>[2x]ADPEVRRCSEQRCPAPYEICPEDYLMSMVWKRTPAGDLAFNQCPLNATGTTSRRCSLSLHGVAFWEQPSFARCISNEYRHLQHSI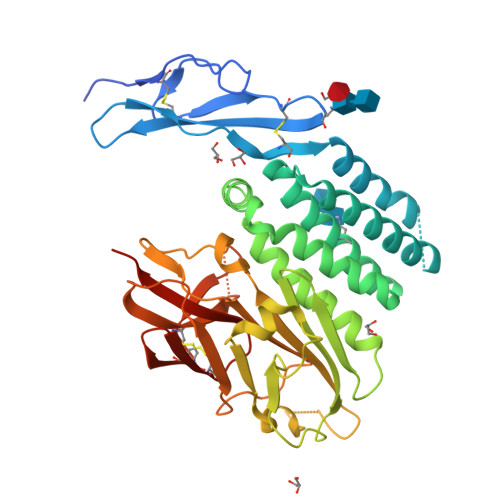KEHLAKGQRMLAGDGMSQVTKTLLDLTQRKNFYAGDLLMSVEILRNVTDTFKRASYIPASDGVQNFFQIVSNLLDEENKEKWEDAQQIYPGSIELMQVIEDFIHIVGMGMMDFQNSYLMTGNVVASIQKLPAASVLTDINFPMKGRKGMVDWARNSEDRVVIPKSIFTPVSSKELDESSVFVLGAVLYKNLDLILPTLRNYTVINSKIIVVTIRPEPKTTDSFLEIELAHLANGTLNPYCVLWDDSKTNESLGTWSTQGCKTVLTDASHTKCLCDRLSTFAILAQQPREHHHHHHHH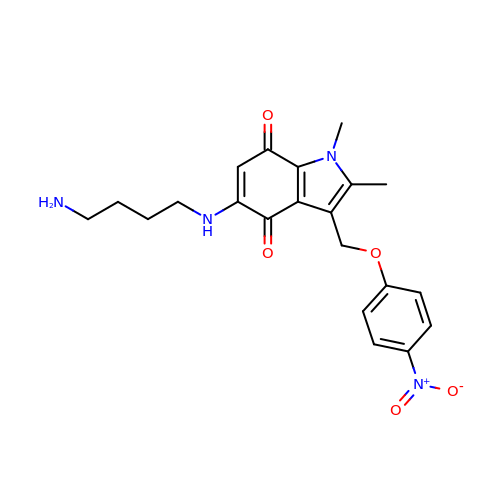5-[(4-aminobutyl)amino]-1,2-dimethyl-3-[(4-nitrophenoxy)methyl]-1H-indole-4,7-dione | C21 H24 N4 O5 | VZTIVOFFCAESGN-UHFFFAOYSA-N> MHLHISSIPHRNSNNSKGGVLDATGPMLSAKRGALLLQAYHRPGEVISYKAGDYHLVPKKFTVGKRIAVRSYLDRNRTELSDRTFMPQKNWFRPYDLQDGCFDRDHERLSYRFYNLETKVIWKAFDTPELIGMLLHDET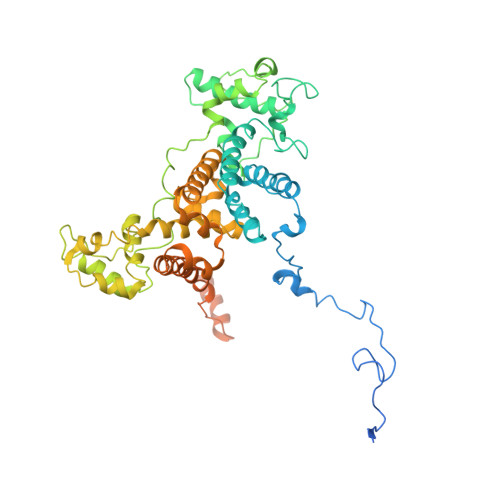VKGNSGMYAPDMLDAALHYTREARYWRCIGITKPFYDRNTLRAHCWEDNGLQVGTLVMSQAMRHALMDLERAVRRKELGLEPNYLWDRWGPIGFIDGARADYLPRFEHNPYVDPDGVDVTEIDVLPFNTHEQIRERYRDFIEPDTAPFEEVFRSPSHGSLTTLADIPNASVVALYKDLKLKAGTPVAGDAVELAPADVRTLFYLSANPEWRAVADGKASWEEVVDAMQPVQAELDEKIDAARLLQNTRHNAERVRAFFEEKCGFHDFMYTPDKTITAAVLCYLTELRRICTETAWGAALAKCLTDMERVQGMGRDAFLVYRHIEDAILDKKRRLWAGRFAGESHEESTLDYLLENFGRRAERPRNVGTTGVEFDREQEPIGRQVQRRVLDSDKANKLAEIRRSRGKMWSKKRSVFDALHEKQLQNFNYGVH> MAYSWSEQVVPSGTTLISVDIEYLDKSYIYLYI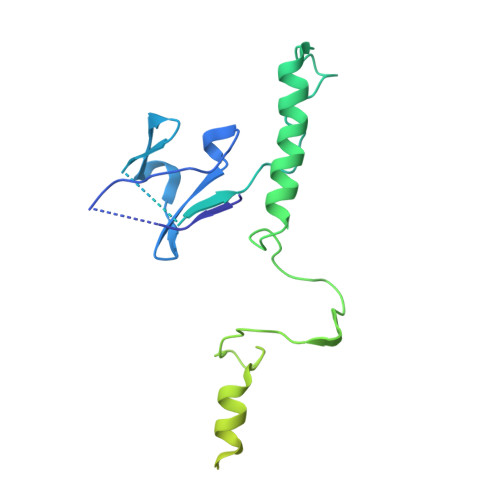NNVLISNSDYSWNSDTLIQLNTPMASAGTVLLVRRTDKEYLYIMFAEGAAFIRENLDVQNTQFLHLAQELVEGRSIDGFYGDLSMNGYRITHLADGVDPKDAVNKGQLDSVSNRVSSIENSFLGLTTVSYPWYTVVSADTDTFEPPFKFTKAALYIDGLCQVPDYSYVVVDNKLLLAESVPTGTVVFARLGEDTDAATEAATTTALAAVQADLQNQINALRALLQGG The present study is devoted to the PA-IIL lectin from Pseudomonas aeruginosa, an opportunistic human pathogen capable of causing lethal complications in cystic fibrosis patients. The lectin may play an important role in the process of virulence, recognizing specific saccharide structures and subsequently allowing the bacteria to adhere to the host cells. It displays high values of affinity towards monosaccharides, especially fucose – a feature caused by unusual binding mode, where two calcium ions participate in the interaction with saccharide. Briefly, the structure is tetrameric with each monomer characterized by a binding site containing two calcium ions and a saccharide.

Hence, amongst the four monomers that form the asymmetric unit, substitution of the sugar occurred in the four monomers of PA-IIL S23A/Me-α-Fuc and G24N/Me-α-Man, but only in three monomers of the S22A/Me-α-Man and S22A/Me-α-Fuc complexes and in only two monomers of G24N/Me-α-Fuc. In case of serine at position 22, the hydroxyl group of the serine side chain is able to make a hydrogen bond with the carboxyl group of Asp96. When this serine is mutated to alanine, the hydroxyl group at 22 is absent and the side chain of Asp96 interacts with a water molecule. Previous work regarding the comparison of PA-IIL and RS-IIL has hinted that the reason behind the different affinities may be in the composition of the specificity binding loop. These observations are further confirmed by the results of the current experiments that point to a very special role for Ser22. In the absence of the side-chain hydroxyl group (mutant S22A), there is no hydrogen bond to Asp96 and the available carboxyl group of Asp96 binds a water molecule. This is in accordance with the observed entropy penalty. The S22A mutant displays a significant drop to a mere 11% of the PA-IIL affinity, its dissociation constant being consequently almost ten fold higher (3.96μM). Overall, the S22A mutant can be described as both fucose- and mannose- binding.

>MATQGVFTLPANTRFGVTAFANASGTQTVNVLVNNETAATFSGQSTNNAVIGTQVLNSGSSGKVQVQVSVNGRPSDLVSAQVILTNELNFALVGSEDGTDNDYNDAVVVINWPLG[4x]>[12x]MSSTILVIHGPNLNLLGKREPEVYGHLTLDNINRQLIAQAEQASITLDTFQSNWEGAIVDRIHQAQTEGVKLI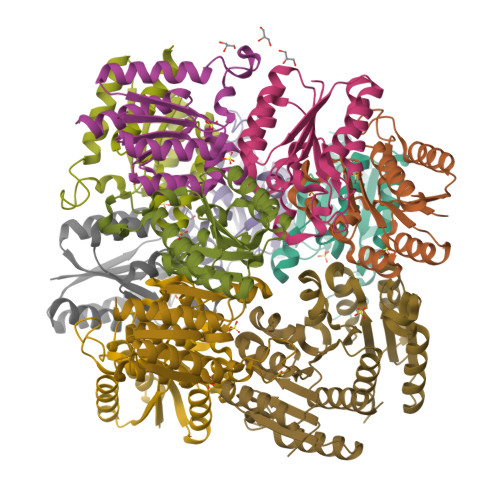IINPAALTHTSVALRDALLGVAIPFIEVHLSNVHAREAFRHHSYLSDKAIGVICGLGAKGYSFALDYAIEKIQPSNPN> MSTKAEQFASKIRYLQEYHNRVLHNIYPVPSGTDIANTLKYFSQTLLSVLRDAPSERGPQSRDAQLSDYPSLDYQGLYVTLVTLLDLVPLLQHGQHDLGQSIFYTTTCLLPFLNDDVLSTLPYTMISTLATFPPFLHKDIIEYLSTSFLPMAILGSSGREGVPAHVNLSASSMLMIAMQYTSNPVYHCQLLECLMKYKQEVWKDLLYVIAYGPSQVKPPAVQMLFHYWPNLKPPGAISEYRGLQYTAWNPIHCQHIECHNAINKPAVKMCIDPSLSVALGDKPPPLYLCEECSERISGDHSEWLIDVLLPQAEISAICQKKNCSSHVRRAVVTCFSAGCCGRHGNRPVRYCKRCHSNHHSNEVGATAETHLYQTSPPPINTRECGAEELVCAVEAVISLLKEAEFHAEQREHELNRRRQLGLSSSHHSLDNTDFDNKDDDKHDQRLLSQFGIWFLVSLCTPSENTPTESLARLVAMVFQWFHSTAYMMDDEVGSLVEKLKPQFVTKWLKTVCDVRFDVMVMCLLPKPMEFARVGGYWDKSCSTVTQLKEGLNRILCLIPYNVISQSVWECIMPEWLEAIRTEVPDNQLKEFREVLSKMFDIELCPLPFSMEEMFGFISCRFTGYPSTVQEQALLWLHVLSELDITVPLQLLISMFSDGVNSVKELANQRKSRANELAGNLASRRVSVASDPGRRGQHNTLSPFHSPFQSPFRSPMRSPFRSPFKNFGHPGGRTIDFDCEDDDMNLNCFILMFDLLLKQMELQDDGITMGLEHSLSKDIISIINNVFQAPWGGSHSCQKDKKATECNLCQSSILCYQLACELLERLAPKEESRLVEPTDSLEDSLLSSRPEFILGPEGEEEENPAAKHGENPGNRTVPSEHAAIKNDTERKFCYQQLPVTLRLIYTIFQEMAKFEEPDILFNMLNCLKILCLHGECLYTARKDHPQFLAYIQDHMLIASLWRVVKSEFSQLSSLAVPLLLHALSLPHGADIFWTIINGNFNSKDWKMRFEAVEKVAVICRFLDIHSVTKNHLLKYSLAHAFCCFLTAVEDVNPAVATRAGLLLDTIKRPALQGLCLCLDFQFDTVVKDRPTILSKLLLLHFLKQDIPALSWEFFVNRFETLSLEAQLHLDCNKEFPFPTTITAVRTNVANLSDAALWKIKRARFARNRQKSVRSLRDSVKGPAESKRALSLPET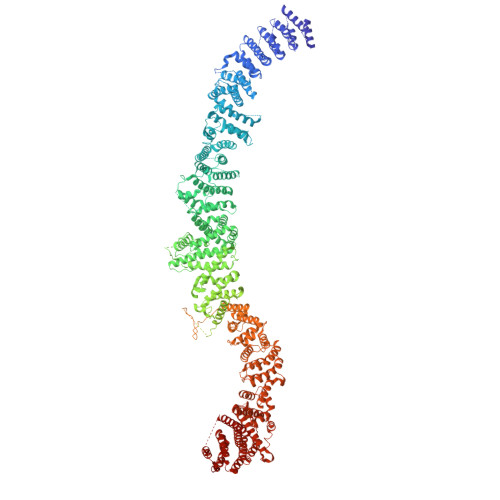LTSKIPVRLTRHEQSAPALGGTPEQTPGQQSPENDNTIKDLLPEDAGIDHQTVHQLITVLMKFMARDESSAESDISSAKAFNTVKRHLYVLLGYDQQEGCFMIAPQKMRLSTCFNAFIAGIAQVMDYNINLGKHLLPLVVQVLKYCSCPQLRHYFQQPPRCSLWSLKPHIRQMWLKALLVILYKYPYRDCDVSKTLLHLIHITVNTLNAQYHSCKPHATAGPLYTDNSNISRYSEKEKEEDSVFDESDIHDTPTGPCNKESQTFFARLKRIGGSRMVKGQPVGMNVQRSEIELAEYRETGALQDSVLHCVREESIQKKKLRSLKQKSLDIGNADSLLFTLDEHRRKSCIDRCDIDKPPAQAAYISQRQNDHHGRSRQNSATRPDNTEIPKNPGTEGFQEIRRPVIPEVRLNCMETFEVRVDSPGKPAPREDLDLIDLSSDSTSGPEKHSILSTSDSDSLVFEPLPPLRIVESDEEEEMMNQGNGGALGNNAASSPSIPSQPSVLSLSTTPLVQVSVEDCSKDFSSKDSGNHQSASNEDSTIAALDDLTDSEELSKSEELREFASGSPLTLKQKRDLLQKSSAVPEMSVDYNPEPSPAEEKPGQTPTSGVKTVLLKVPEDGENLIESEKPNTSAESDTEQNPERKVEEDGAEESEFKIQIVPRQRKQRKIAVSAIQREYLDISFNILDKLGEQKDPDPSAKGLSTLEMPRESSSAPTLEAGAPETSSHSSISTQYRQMKRGSLGVLTMSQLMKRQLEHQSSAPHNISSWDTEQIQPGKRQCNVPMCLNPDLEGQPLRTRGATKSSLLSAPSIASMFVPAPEEFTEEQPTVMADKCHDCGAILEEYDEETLGLAIVVLSTFIHLSPDLAAPLLLDIMQSVGRLASSTTFSNQAESMMVPGNAAGVAKQFLRCIFHQLAPNGIFPQLFQSAIKDGTFLRTLATSLMDFNELSSIAALSQLLEGLNNKKNLPAGGAMIRCLENIATFMEALPMDSPSSLWTTISNQFQTFFAKLPCVLPLKCSLDSSLRIMICLLKIPSTNATRSLLEPFSKLLSFVIQNAVFTLAYLVELCGLCYRAFTKERDKFYLSRSVVLELLQALKLKSPLPDTNLLLLVQFICADAGTKLAESTILSKQMIASVPGCGTAAMECIRQYVSEVLEFMADMHTLTKLKSHMKTCSQPLHEDTFGGHLKVGLAQIAAMEISRGNHRDNKAVIRYLPWLYHPPSAMQQGPKEFIECVSHIRLLSWLLLGSLTHNAVCPNASSPCLPIPLDAGSHIADHLIVILIGFPEQSKTCVLHMCSLFHAFIFAQLWTVYCEQSAVATNVQNQNEFSFTAILTALEFWSRVTPSILQLMAHNKVMVEMVCLHVISLMEALQECNSTIFVKLIPMWLPMIQSNTKHLSAGLQLRLQAIQNNVNHHSLRTLPGSGQSSAGLAALRKWLQCTQFKMAQVEIQSSEAASQFYPL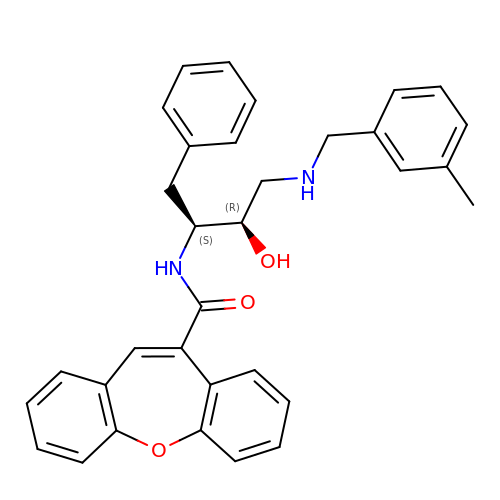N-{(1S,2R)-1-BENZYL-2-HYDROXY-3-[(3-METHYLBENZYL)AMINO]PROPYL}DIBENZO[B,F]OXEPINE-10-CARBOXAMIDE | C33 H32 N2 O3 | BNWZCXDHHPBQOX-XZWHSSHBSA-N>GSSSGAAGLSGLHRTYSQDCSFKNSMYHVGDYVYVEPAEANLQPHIVCIERLWEDSAGEKWLYGCWFYRPNETFHLATRKFLEKEVFKSDYYNKVPVSKILGKCVVMFVKEYFKLCPENFRDEDVFVCESRYSAKTKSFKKIKLWTMPISSVRFVPRDVPLP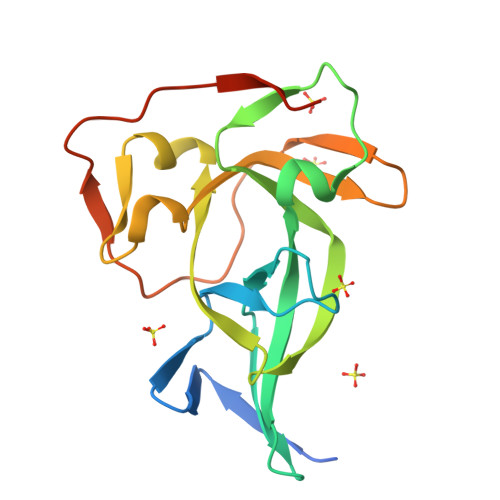VVRVASVFANADGNS[6x]> GCGCCUGGACUUAAAGCCAUUGCACU;> CCGGCUUUAAGUUGACGAGGGCAGGGUUUAUCGAGACAUCGGCGGGUGCCCUGCGGUCUUCCUGCGACCGUUAGAGGACUGGUAAAACCACAGGCGACUGUGGC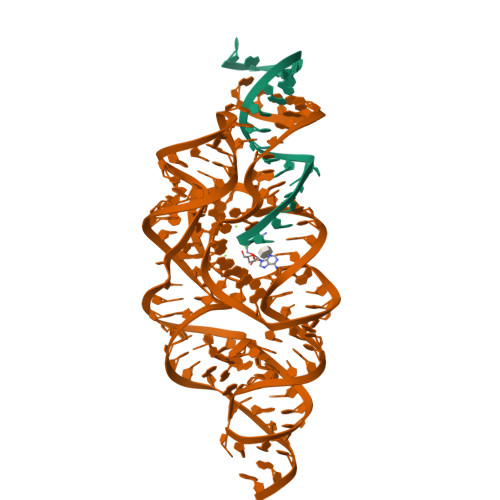AUAGAGCAGUCCGGGCAGGAA> MYIEMAQQQQQSGSDNSMAPVWIVILLFITAYFVWALAHQYIVSFVFTINIWQARLVNLFLNNQLLANQIYLMQTLDPNTVNWDQMVTVMRAVGDYMRYPVICILVVLAFVLYNSNVTLKYRKTYDMKSLRAQEQFNWPAIMPIVKEDLVSQDVNKGPWAMALTPMEFARKYNLLRKDDALLDNPVPGEEMTAGIRRGDAKRVFTMQLGPYWDGFERCSPQAYALSAVFMARMNRDRDAANNILKVLDKTFVDGKPDFSVARPVMKKYQNSELVQEVVAKHAYVLTVIASLLEAAREDGVVPSSEFLWLKPVDRRLWYMLNCVGRQTPYSEVAGPFAHWKAEKEMGRRSLVPMIDEAIRALEIAVKEVRLT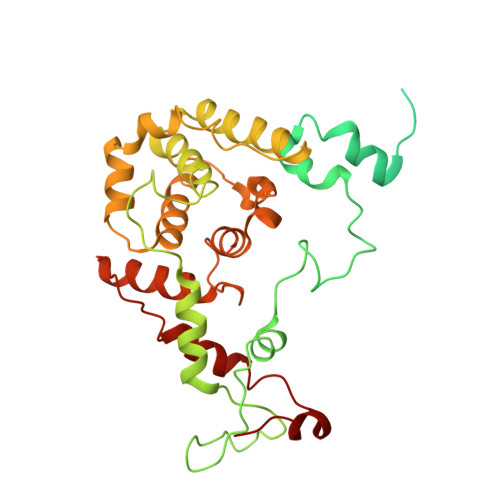PRQMEELEP Penicimutamide 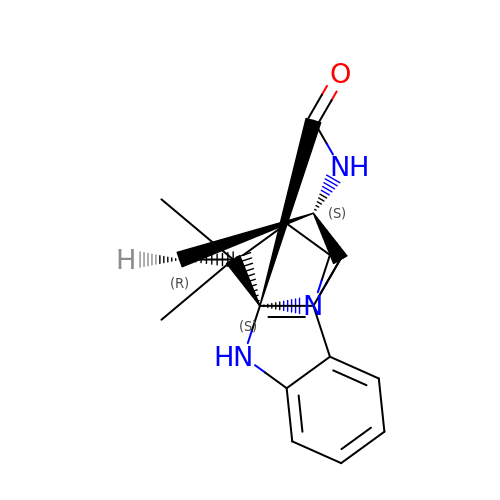E  | C21 H25 N3 O | LBTZXCFDJFHPMI-HBGVWJBISA-N> GGCGCGAGGAA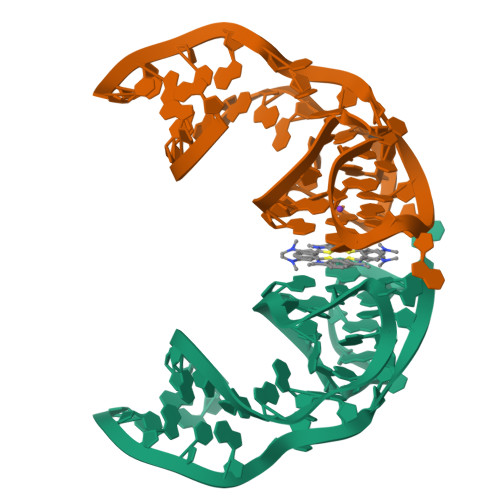GGUGGUCUGAGGAGGUCACUGCGCC> MSIFTIFISALLVNNFVLSRFLGICPFLGVSKKVETATGMGAAVTFVMALAAIMTFLVERFILIPLNIQYLSTLAFILVIASLVQFVEMVIKKVSPDLYKALGIYLPLITTNCAVLGMAVINSNEKYNLIQSIINSVGAALGFTLALVLLAGIREKMETNEYIPEALKGLPITLVTAGLMAIAFLGFQGLI;> MEGLLFPVLSLGGLGVVFGLLLGYASKKFAVEVDERVPMVRAALPGANCGGCGFAGCDAYADAVVNAGAKPNGCPVGGAACAAKIAEIMGVVVDSSEPKKAYVKCQGTCDKAKEKYEYYGA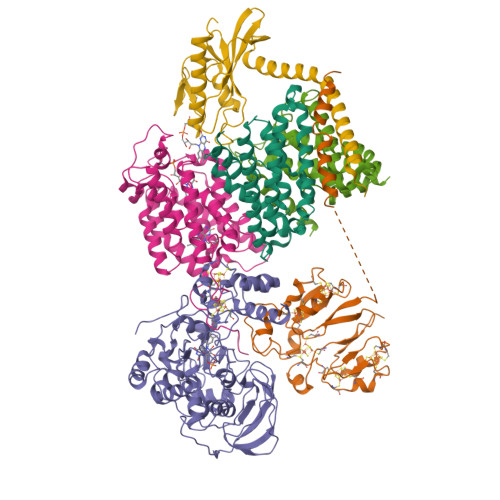MTCVDAANIPGAGSKTCGFGCLGLGSCVQVCAFDAIHVENGIAVVDEEACTGCGACVSICPKSVIELTPMSKKVRISCNSHDKGIEVKNACSVGCLSCGLCVRNCPSEAITMVNNLPVIDYDKCTQCGVCVGKCPTKAIVNLNTNVSKEASNN;> MELLTFKNGVHPPHGKHYTENKPIEEYLPKGDIVIPMSQHIGAPAEPIVKKGDRVLVGQKIGEAKGFVSANIHASVSGTVKNVAPVTLFNGVKSTAVIIENDGQYEEIETEKRDYTKLSNEEIINIIKEAGIVGMGGATFPTHVKLAPPPDKNIDSIVVNAAECEPYLTCDHRMMLEKTNEIVEGLKIVLKLFPKATGYIGIEDNKMNAIKAMQEAVKNIANIEVKAVKTKYPQGAEKQLIYAITKREVPSGGLPADAGCIVQNVDTIYEIYNAVVNGKPLTSRVVTVTGDAIKEPKNLRFKIGTSVRELVEAAGGFAEEPLKVISGGPMMGMAMYSLDVPSTKGTSGVLCLTKKVAEIEEESNCINCGKCVQVCPMNLMPTKLATASAVSNLDMFNEFSGRDCIECGCCSFVCPARRHLLQRIRSGKKAVSKKK;> MSETTMYTVSSSPHIRAKDTTQSIMRDVVIALLPATIAGVYFFKLQGLLVILASVLSCVVAEYIWQKASKKKVTVGDYSAVVTGLLLAFNVPASIPLWIPVVGGFFAIIVVKQFFGGLGQNIVNPALAARAFLLASWPVQMTSWTLDGVTTATPLAILKGNEATGAAAPDLMSVFIGHVGGCIGETSALALLIGGAYLFYKHIIDWRIPVSFIGTTFIFTAIAGRGSSPVYELFAGGLMLGAIFMATDYATSPITPLGRIIFGVGCGVITSLIRIFGGYPEGVSYSILVMNLFVPLIERWTAPKIFGKVK;> MGVVSERLYNGIVKENATFVQVLGMCPTLAVTTSAINGIGMGLSATVVLIGSNVVISLLKKVIPDEIRIPAYITVIATLVTVLQFLLQAYLPDLNKSLGIFIPLIVVNCIILGRAEAYANKNSVGASFFDGLGMGLGFTVSLAALGIIREFLGTGKVFGAQITPDAFQPALIMILAPGGFFTLGILMAILNQRKLKKAKAK;> MKKVSSFKLGMVLLLIAAVCGLILGGVNQVTAEPIAIQNKKTLDEANKAILPEASEFAEKTDIKGEGIVLGVTEGKSGSDLKGYTIKVAPKGYAGAIEMMVGVSTEGKVTGIKILNHAETPGLGANATDPKFSGQYANKPAKELKVVKGAASGEDEIVAITGATITSKAVTLGVNEAIKFYDTKLKGGK> SILYAGPTFTHSPAASNLPI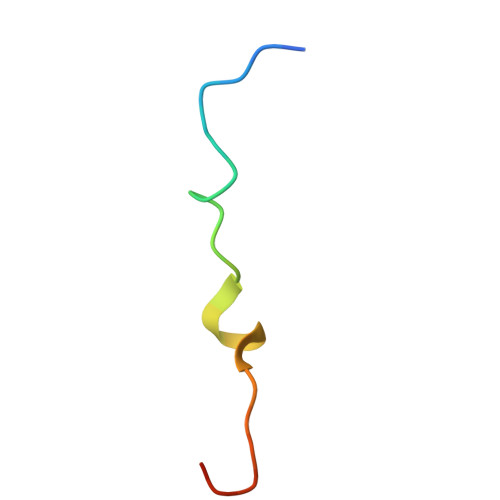PTFLHS>SNAMKHYLICFDVQHDKTRAKLSRLLEKYGPRVQGSVFEVSFKTPDRKRQLEYKIHQIIKQSNTEENNIRFYNLNKDTIKHSHDINGNPIAQLPAAIVL[2x];>SNAMILPSFPDLTGLVVNLKFTARAEFSLNHEMAVDAFLRHSLNLGESYSHHLSIITPENGRLFYREGDTYRFVVIAMGNQQQTNSIWHTLINHLRKLPDSAPITDKQAPLRNNIKLESLNDLFDGIPVSSKESLDAYTLQRAMEQGLAWHKAANLTEQPLDIQWYWQSTVRILHADHKQHKGEQRYCRDAVQLTPLLLLKRIYETLNNVATYFGLKTNKNTTENHQAWLKEQAQYIEIQHPDLYWIDTPYFGKDAEKNTLGGMAGNFTLSLKPGIEPGLLAMLILTQMVGVGQRRTSGLGKYWLKHSLKHAHLILGLKPNRVTRSQTLLDCIIQPHIISQAIAEIEKKTNI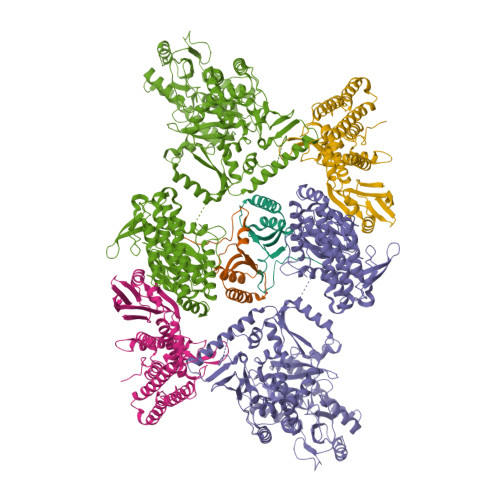DTLNERTLSQVQSAIGQLRKHQYQAPKLQGFTIPKKDGTERLLAVSPLYDRILQKAAAIVLTPGLDAIMSQASYGYRKGLSRQQVRYEIQNAYRQGYHWVYESDIEDFFDAVYRPQLINRLKSLLGNDPLWEQIESWLGQDIHIKDTIIERTPNLGLPQGSPLSPLLANFILDDFDSDLETHGFKIIRFADDFIILCKSQHEAQQAAHAVEQSLKEVKLSINVEKTHIIQLNQGFRFLGYLFREDHAIEIAGEKSDGRTTFAAEQTPTNLPPWLANLGTKSPQPLADDDLPKKSYGQIETQGTHLVLAGDAQIITTDNQNLIVKKDDKITHKISLEQLHAVTLIGLHTMTLPAKHRLLEHKIPVHIADRTGRYLGAVTSFQPAQNNYKNWFIQLQMCDREPFAHAIAQQIVISRIHNQRQTLLKRKAHRKQLQQTLSNLKKLQYKVTAATKRSSLNGLEGSATREYFQQFNLFLPEWAHFSKRTRRPPKDPFNVLLSLGYTILYSHTDAILQSAGFITWKGIYHQQSAAHAALASDIMESYRHLVERYAIYIINHGQIKQDDFRQEKDHLGQDTIRLSAEARRRYVGGLINRFQKFSKDKTLHQHLYQQAQQLKNAMHNQQSSQFQVWKELK[4x]>[2x]MANQISLPRLVDLDWRVDIKT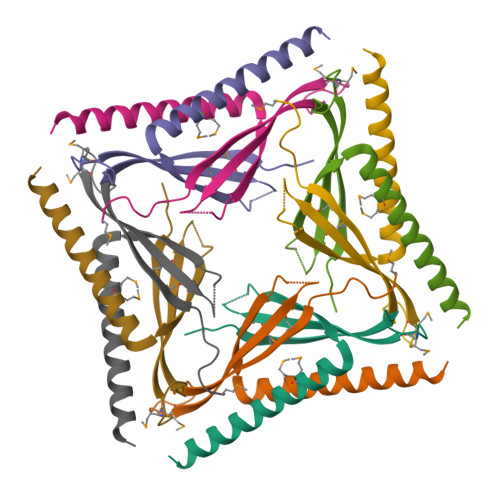SSDSISRMAVPTCLLQMKIQEDPSLCGDKPSISAVTVELSKETLDTMLDGLGRIRDQLSAVASKLEHHHHHH>[2x]MGSSHHHHHHSQDPMTDSTTHYTRPDVAAFLAFLNAQEGPKMEEMPPAGAREMMRVMGQLADVPRGEIAKVEDRMIPGPDGDIPIRLYDNRPDREAGPVMVFYHGGGWVIGDLETHDPYCAEAARILDMPVIAIDYRLAPEHPFPAAPIDCEAATRWVADNIACTGLVLSGDSAGGNLTIVTALALRDEPAAKPVIAIHPIYPAVTTHNDWQSYRDFGEGHLLTEGSMTWFGNHYAADPADRRAAPIDFPADGLPPTLLITASLDPLRDQGRAYAAKLIEAGVPTTYREAKGTIHGYICLAQGIPSAKDDIRGALTVLKAIVAEATGAA

Herein, we identified from a library of lipases/esterases/acyltransferases and variants thereof a lipase originating from Sphingomonas sp. HXN-200 (SpL) able to form amides in aqueous solution starting from a broad scope of sterically demanding heteroaromatic ethyl esters as well as aliphatic amines, reaching isolated yields up to 99% on preparative scale and space time yields of up to 864 g L–1 d–1; thus, in selected cases, the amide was formed within minutes. SpL is a hormone-sensitive lipase-like (HSL-like) protein adopting the alpha-beta hydrolase fold, with a helical lid domain over the active site cavity with the catalytic triad. The common Ser-His-Asp catalytic triad was located at positions Ser159, His281, and Asp251. Mutational and structural studies revealed that an aspartate next to the catalytically active serine is highly beneficial for the observed activity, which has not been described before, showing that a catalytic tetrad is actually required (Asp-Ser-His-Asp) for SpL for efficient amide formation in aqueous buffer.

Diffraction data were collected under cryo-conditions from native crystals, as well as from crystals soaked with benzylamine 2a or the amide N-benzyl-2-pyridinecarboxamide 3a,a leading to data sets with resolutions of 2.0, 1.6, and 1.8 Å, respectively. In the complex with benzylamine, three benzylamine molecules (ABN1–3) could be placed into the electron density in the active site. ABN3 was located in the nucleophile channel and adopts a position from which a nucleophilic attack on an assumed enzyme-acyl intermediate can be facilitated and is therefore considered at the catalytically relevant nucleophile position. Next to Ser159 of the catalytically active triad, an aspartate (Asp158) caught our attention as it is not present, e.g., in the lipase from C. antarctica B (CalB). Thus, a carboxylic acid moiety next to the serine at the binding site of the amine in the structure seems highly beneficial for amide formation. As Asp158 in SpL seemed to be of high relevance for efficient amide formation, and putatively the negative charge of Asp158 is important to set the microscopic electrostatic environment at this position in favor of amide formation, we hypothesize that its carboxylate moiety may support deprotonation of the positively charged protonated amine substrate in buffer, which cannot act as a nucleophile. By ensuring deprotonation of the aminium species, the amine becomes available as a nucleophile, which can then attack the acyl-enzyme intermediate following the classical lipase mechanism.> GEFAAARESERQLRLRLCVLNEILGTERDYVGTLRFLQSAFLHRIRQNVADSVEKGLTEENVKVLFSNIEDILEVHKDFLAALEYCLHPEPQSQHELGNVFLKFKDKFCVYEEYCSNHEKALRLLVELNKIPTVRAFLLSCMLLGGRKTTDIPLEGYLLSPIQRICKYPLLLKELAKRTPGKHPDHPAVQSALQAMKTVCSNINETKRQMEKLEALEQLQSHIEGWEGSNLTDICTQLLLQGTLLKISAGNIQERAFFLFDNLLVYCKRKSRVTGSKKSTKRTKSINGSLYIFRGRINTEVMEVENVEDGTADYHSNGYTVTNGWKIHNTAKNKWFVCMAKTAEEKQKWLDAIIREREQRESLKLGMERDAYVMIAEKGEKLYHMMMNKKVNLIKDRRRKLSTVPKCFLGNEFVAWLLEIGEISKTEEGVNLGQALLENGIIHHVSDKHQFKNEQVMYRFRYDDGTYKARSELEDIMSKGVRLYCRLHSLYTPVIKDRDYHLKTYKSVLPGSKLVDWLLAQGDCQTREEAVALGVGLCNNGFMHHVLEKSEFRDESQYFRFHADEEMEGTSSKNKQLRNDFKLVENILAKRLLILPQEEDYGFDIEEKNKAVVVKSVQRGSLAEVAGLQVGRKIYSINEDLVFLRPFSEVESILNQSFCSRRPLRLLVATKAKEIIKIPDQPDTLCFQIRGAAPPYVYAVGRGSEAMAAGLCAGQCILKVNGSNVMNDGAPEVLEHFQAFRSRREEALGLYQWIYHTHEDAQEARASQEASTEDPSGEQAQEEDQADSAFPLLSLGPRLSLCEDSPMVTLTVDNVHLEHGVVYEYVSTAGVRCHVLEKIVEPRGCFGLTAKILEAFAANDSVFVENCRRLMALSSAIVTMPHFEFRNICDTKLESIGQRIACYQEFAAQLKSRVSPPFKQAPLEPHPLCGLDFCPTNCHINLMEVSYPKTTPSVGRSFSIRFGRKPSLIGLDPEQGHLNPMSYTQHCITTMAAPSWKCLPAAEGDPQGQGLHDGSFGPASGTLGQEDRGLSFLLKQEDREIQDAYLQLFTKLDVALKEMKQYVTQINRLLSTITEPTSGGSCDASLAEEASSLPLVSEESEMDRSDHGGIKKVCFKVAEEDQEDSGHDTMSYRDSYSECNSNRDSVLSYTSVRSNSSYLGSDEMGSGDEL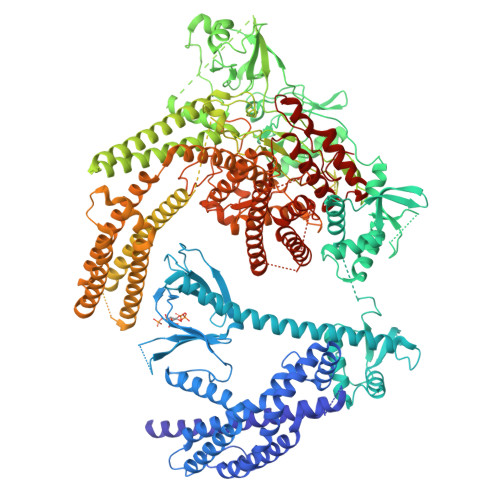PCDMRIPSDKQDKLHGCLEHLFNQVDSINALLKGPVMSRAFEETKHFPMNHSLQEFKQKEECTIRGRSLIQISIQEDPWNLPNSIKTLVDNIQRYVEDGKNQLLLALLKCTDTELQLRRDAIFCQALVAAVCTFSEQLLAALGYRYNNNGEYEESSRDASRKWLEQVAATGVLLHCQSLLSPATVKEERTMLEDIWVTLSELDNVTFSFKQLDENYVANTNVFYHIEGSRQALKVIFYLDSYHFSKLPSRLEGGASLRLHTALFTKVLENVEGLPSPGSQAAEDLQQDINAQSLEKVQQYYRKLRAFYLERSNLPTDASTTAVKIDQLIRPINALDELCRLMKSFVHPKPGAAGSVGAGLIPISSELCYRLGACQMVMCGTGMQRSTLSVSLEQAAILARSHGLLPKCIMQATDIMRKQGPRVEILAKNLRVKDQMPQGAPRLYRLCQPPVDGDL> MKLPLLLALLFGAVSALHLRSETSTFETPLGAKTLPEDEETPEQEMEETPCRELEEEEEWGSGSEDASKKDGAVESISVPDMVDKNLTCPEEEDTVKVVGIPGCQTCRYLLVRSLQTFSQAWFTCRRCYRGNLVSIHNFNINYRIQCSVSALNQGQVWIGGRITGSGRCRRFQWVDGSRWNFAYWAAHQPWSRGGHCVALCTRGGHWRRAHCLRRLPFICSY;>[2x]REARGATEEPSPPSRALYFSGRGEQLRLRADLELPRDAFTLQVWLRAEGGQRSPAVITGLYDKCSYISRDRGWVVGIHTISDQDNKDPRYFFSLKTDRARQVTTINAHRSYLPGQWVYLAATYDGQFMKLYVNGAQVATSGEQVGGIFSPLTQKCKVLMLGGSALNHNYRGYIEHFSLWKVARTQREILSDMETHGAHTALPQLLLQENWDNVKHAWSPMKDGSSPKVEFSNAHGFLLDTSLEPPLCGQTLCDNTEVIASYNQLSSFRQPKVVRYRVVNLYEDDHKNPTVTREQVDFQHHQLAEAFKQYNISWELDVLEVSNSSLRRRLILANCDISKIGDENCDPECNHTLTGHDGGDCRHLRHPAFVKKQHNGVCDMDCNYERFNFDGGECCDPEITNVTQTCFDPDSPHRAYLDVNELKNILKLDGSTHLNIFFAKSSEEELAGVATWPWDKEALMHLGGIVLNPSFYGMPGHTHTMIHEIGHSLGLYHVFRGISEIQSCSDPCMETEPSFETGDLCNDTNPAPKHKSCGDPGPGNDTCGFHSFFNTPYNNFMSYADDDCTDSFTPNQVARMHCYLDLVYQGWQPSRKPAPVALAPQVLGHTTDSVTLEWFPPIDGHFFERELGSACHLCLEGRILVQYASNASSPMPCSPSGHWSPREAEGHPDVEQPCKSSVRTWSPNS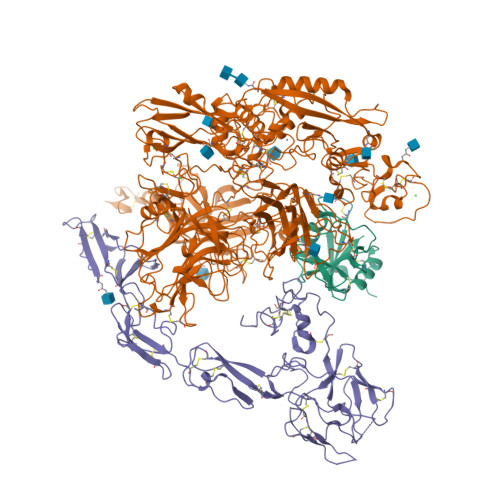AVNPHTVPPACPEPQGCYLELEFLYPLVPESLTIWVTFVSTDWDSSGAVNDIKLLAVSGKNISLGPQNVFCDVPLTIRLWDVGEEVYGIQIYTLDEHLEIDAAMLTSTADTPLCLQCKPLKYKVVRDPPLQMDVASILHLNRKFVDMDLNLGSVYQYWVITISGTEESEPSPAVTYIHGSGYCGDGIIQKDQGEQCDDMNKINGDGCSLFCRQEVSFNCIDEPSRCYFHDGDGVCEEFEQKTSIKDCGVYTPQGFLDQWASNASVSHQDQQCPGWVIIGQPAASQVCRTKVIDLSEGISQHAWYPCTISYPYSQLAQTTFWLRAYFSQPMVAAAVIVHLVTDGTYYGDQKQETISVQLLDTKDQSHDLGLHVLSCRNNPLIIPVVHDLSQPFYHSQAVRVSFSSPLVAISGVALRSFDNFDPVTLSSCQRGETYSPAEQSCVHFACEKTDCPELAVENASLNCSSSDRYHGAQCTVSCRTGYVLQIRRDDELIKSQTGPSVTVTCTEGKWNKQVACEPVDCSIPDHHQVYAASFSCPEGTTFGSQCSFQCRHPAQLKGNNSLLTCMEDGLWSFPEALCELMCLAPPPVPNADLQTARCRENKHKVGSFCKYKCKPGYHVPGSSRKSKKRAFKTQCTQDGSWQEGACVPVTCDPPPPKFHGLYQCTNGFQFNSECRIKCEDSDASQGLGSNVIHCRKDGTWNGSFHVCQEMQGQCSVPNELNSNLKLQCPDGYAIGSECATSCLDHNSESIILPMNVTVRDIPHWLNPTRVERVVCTAGLKWYPHPALIHCVKGCEPFMGDNYCDAINNRAFCNYDGGDCCTSTVKTKKVTPFPMSCDLQGDCACRDPQAQEHSRKDLRGYSHG> ALMITDECINCDGCEPECPNGAISQGDETYVIEPSLCTECVGHYETSQCVE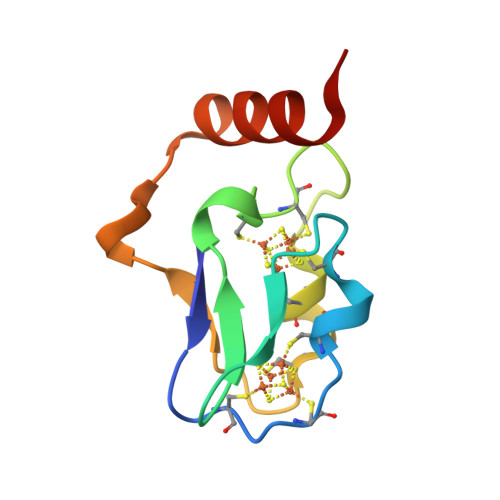VCPVDCIIKDPSHEETEDELRAKYERITGEG> GSIISCSAQSVTADPSPPITDTNKLNKYSSRITEPKSQGGSQAILHGVGLSDDDLLKPQIGISSVWYEGNTCNMHLLKLSEAVKEGVENAGMVGFRFNTIGVSDAISMGTRGMCFSLQSRDLIADSIETVMSAQWYDGNISIPGCDKNMPGTIMAMGRLNRPGIMVYGGTIKPGHFQDKTYDIVSAFQSYGEFVSGSISDEQRKTVLHHSCPGAGACGGMYTANTMASAIEAMGMSLPYSSSIPAEDPLKLDECRLAGKYLLELLKMDLKPRDIITPKSLRNAMVSVMALGGSTNAVLHLIAIARSVGLELTLDDFQKVSDAVPFLADLKPSGKYVMEDIHKIGGTPAVLRYLLELGLMDGDCMTVTGQTLAQNLENVPSLTEGQEIIRPLSNPIKETGHIQILRGDLAPDGSVAKITGKEGLYFSGPALVFEGEESMLAAISADPMSFKGTVVVIRGEGPKGGPGMPEMLTPTSAIMGAGLGKECALLTDGRFSGGSHGFVVGHICPEAQEGGPIGLIKNGDIITIDIGAARIDTQVSPEEMNDRRKKWTAPAYKVNRGVLYKYIKNVQSASDGCVTDE

Dihydroxy acid dehydratase (DHAD) is the third enzyme in the plant branched-chain amino acid biosynthetic pathway and the target for commercial herbicide development. We have previously reported the discovery of fungal natural product aspterric acid (AA) as a submicromolar inhibitor of DHAD through self-resistance gene directed genome mining. Here, we reveal the mechanism of AA inhibition on DHAD and the self-resistance mechanism of AstD, which is encoded by the self-resistance gene astD. Our structural and kinetic analysis of the mutant AthDHADs has validated the hypothesis that larger hydrophobic amino acids surrounding the active-site entrance enhance resistance to AA.

In this work, we solved the crystal structure of AthDHAD–AA complex with 2.0-Å resolution, which provides the critical information for the inhibition mechanism at the atomic level. In the dimer structure of AthDHAD and AA complex, the active site is located at the interspace between the N-terminal domain (residues 1 to 388) and the C-terminal domain (residues 394 to 573), formed by 2Fe–2S cluster and Mg2+. AA was observed at the active site and the substrate channel with an occupancy of 0.90. AA fills essentially the entire substrate pocket via polar and hydrophobic interactions. The carboxyl and hydroxyl groups of AA are coordinated with Mg2+. The β-ether oxygen of AA participates in the formation of hydrogen bond networks via W. Hence, the closely positioned [2Fe–2S], Mg2+, W, and the residues T216, E463, and D140 all contribute to anchoring the hydrophilic side of AA in the active site. Extensive hydrophobic interactions between the nonpolar regions of AA and residues that line the substrate entry channel, including M102, I177, V178, F181, Y215, and L465, are observed in the complex structure. Such nonpolar interactions are not possible with either DHI or DHMV and rationalize the strong binding of AA to AthDHAD (Ki ~ 300 nM) as a competitive inhibitor. Binding of AA expanded the active chamber by pushing outward the residues forming the cavity, including residues I177, V178, F181, G490, and E463. The binding of AA moves Mg2+ about 0.7 Å deeper into the pocket and changes the side chain of coordinating residues.>VDQVGVTDFTADKTSAKADGTEAITYTATVKKNGVAQANVPVSFNIVSGTAVLSANSANTNGSGKATVTLKSDKPGQVVVSAKTAEMTSALNANAVIFVDQTKASITEIKADKTTAVANGQDAITYTVKVMKGDKPVSNQEVTFTTTLGKLSNSTEKTDT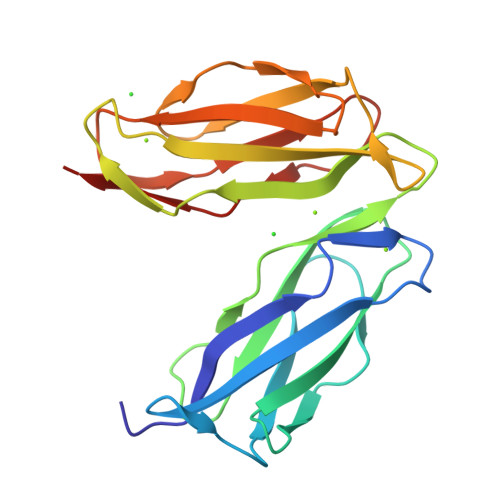NGYAKVTLTSTTPGKSLVSARVSDVAVDVKAPEVEFFTT[2x]>MTYTVGHYLATRLAQIGLKHHFAVAGDYNLVLLDQLLKNKDLEQVYCCNELNCGFSAEGYARANGVGAAVVTFSVGALSAFNAIGGAYAENLPVILISGAPNTNDHGSGHILHHTIGTTDYGYQLEMAKQITCAAVSITHAEDAPALIDHAIRTALREKKPAYIEIACNVAAQPCARPGPVSALLNEPTSDEETLKAAVEAALDFIEKREKPVLLVGGKLRAAGAEEAVVELADALGCAVATMAAAKSFFPEDHPGYVGTYWGEVSSPGVEEIVDWADGIICLGPVFNDYSTVGWTAWPKGENVVLVDPHHITVGGEEFTGIHLKDFLTALTERVPKKDATLDQFKARVGKPAAEKVPAADPNAPLTRAELCRQIQGLLNPNTTLIAETGDSWFNAMRMKLPHGARVELEMQWGHIGWSVPATFGYAVAEPERRNVLMVGDGSFQLTAQEVAQMVRRKLPIIIFLINNRGYTIEVKIHDGPYNNIKNWDYAGLMEVFNAEDGKGLGLKATTGGELAEAIKKALAHREGPTLIECVIDRDDCTPELVTWGKKVATANARPPQAI[4x]

Pyruvate decarboxylase (PDC; EC 4.1.1.1) is a thiamine pyrophosphate- and Mg2+ ion-dependent enzyme that catalyses the non-oxidative decarboxylation of pyruvate to acetaldehyde and carbon dioxide. Bacterial PDCs are key enzymes in homofermentative metabolism where ethanol is the main fermentation product, and as such are of great interest for biotechnological applications, including second-generation bioethanol production for use as a renewable transport fuel. In this study, we employed ASR to infer an ancestral bacterial PDC designated ANC27. Here, we present the crystal structure of the inferred ancestral PDC ANC27 at 3.5 Å resolution, show that the enzyme is fully functional and compare it with known extant bacterial PDCs.

The final model comprises four chains of 563 amino acids with a molecular mass of 60.6 kDa, each with a TPP and an Mg2+ ion, together with one water in the active site of chain A and one PEG molecule between chains A and C. The final model contains four monomers in the asymmetric unit, each comprising part of a dimer formed with a symmetry-related monomer, with the dimers coming together in a less tight interaction to form dimer-of-dimers tetramers. Overall, the electron-density map was of good quality, apart from the N-terminal methionine and the loop 340–360, which is the exposed linker between the R and PP domains. These regions seem to be very flexible and have not been included in the final model (more specifically chain A residues 344–358, chain B residues 343–359, chain C residues 343–357, chain D residues 340–358 and the N-terminal methionine in all chains). There is good-quality electron-density evidence for a TPP molecule and an Mg2+ ion in each of the four chains in the structure. Each TPP binds as indicated by the domain nomenclature, with the pyrophosphate group binding to the PP domain of one monomer and the pyrimidine ring binding to the PYR domain of a second monomer in a dimer, thus creating the active site in a narrow cleft at the interfaces between the two monomers. The O atoms of the pyrophosphate form hydrogen bonds to the backbone amide groups of Ile473 and Thr472, while the N1 atom on the pyrimidine ring forms a hydrogen bond to Glu50 (from the second monomer). The Mg2+ ion anchors the pyrophosphate group of the TPP and forms interactions with the two O atoms on the diphos­phate group of the TPP, the side-chain O atoms of Asp441 and Asn467 and the main-chain O atom of Gly470. Although the ancestral protein ANC27 did not possess the thermostability that we hoped for, the suggestion that the lack of inter-dimer interactions appears to be the cause of its fragility should guide future ancestral reconstruction protocols to achieve the desired characteristics.>[2x]MFDIALYEPEIAPNTGNIIRLCANCGANLHLIEPLGFDLEEKKVRRAGLDYHDLARVTRHKNYQAFLDYLEQRGEYRIFACTTKTTGHHVDAQYRQGDVLLFGPETRGLPMEVIESLPMSQ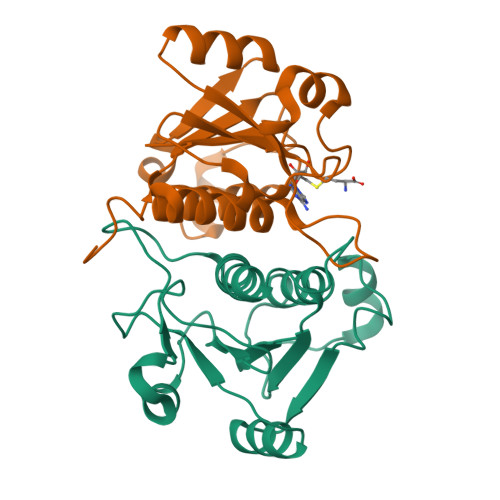RIRIPMMPDARSLNLSNAVAIIAFEAWRQLGFQGAKGHHHHHHG>ENLTPQHMASMALTGTDRVKRGMAEMQKGGVIMDVVNAEQAKIAEAAGAVAVM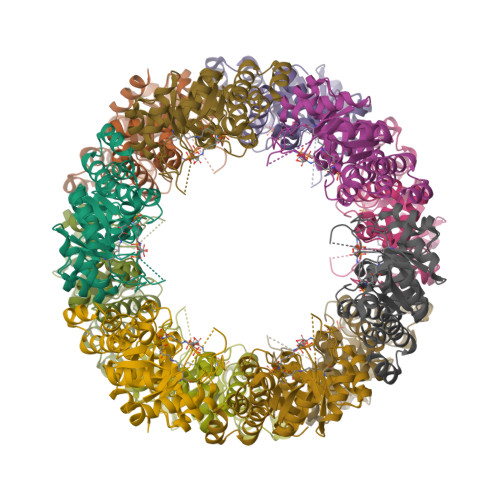ALERVPADIRAAGGVARMADPTVIEEVMNAVSIPVMAXVRIGHYVEARVLEALGVDYIDESEVLTPADEEFHIDKRQFTVPFVCGCRDLGEAARRIAEGASMLRTXGEPGTGNIVEAVRHMRKVNAQIRKVVNMSEDELVAEAKQLGAPVEVLREIKRLGRLPVVNFAAGGVTTPADAALMMHLGADGVFVGSGIFKSENPEKYARAIVEATTHYEDYELIAHLSKGLGGAMRGIDIATLLPEHRMQERGW[6x]> TLDSLARDLTVIAKDGTLDPVIGRDKEITRVIEVLSRRTKNNPVLIGEPGVGKTAIAEGLAQAIVNNEVPETLKDKRVMSLDMGTVVAGTKYRGEFEERLKKVMEEIQQAGNVILFIDELHTLV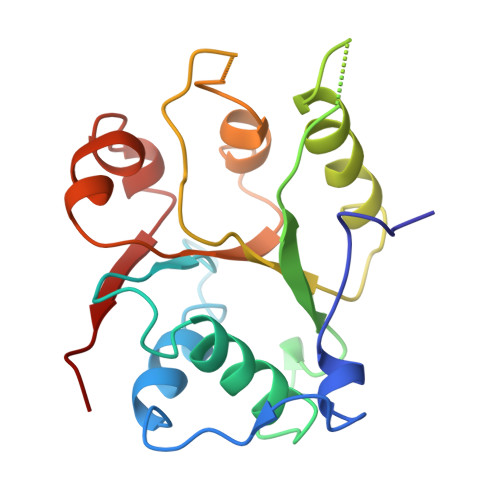GAGGAEGAIDASNILKPALARGELQCIGATTLDEYRKNIEKDAALERRFQPVQVDEP> SHMELTPDQQTLLHFIMDSYNKQRMPQEITNKILKEEFSAEENFLILTEMATNHVQVLVEFTKKLPGFQTLDHEDQIALLKGSAVEAMFLRSAEIFNKKLPSGHSDLLEERIRNSGISDEYITPMFSFYKSIGELKMT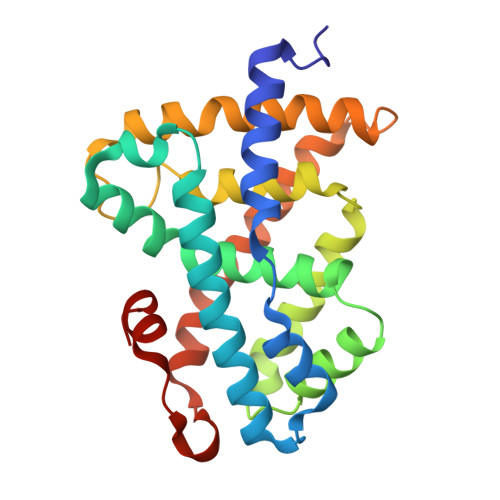QEEYALLTAIVILSPDRQYIKDREAVEKLQEPLLDVLQKLCKIHQPENPQHFACLLGRLTELRTFNHHHAEMLMSWRVNDHKFTPLLCEIWDVQ> MLSIKDLHVSVEDKAILRGLSLDVHPGEVHAIMGPNGSGKSTLSATLAGREDYEVTGGTVEFKGKDLLALSPEDRAGEGIFMAFQYPVEIPGVSNQFFLQTALNAVRSYRGQETLDRFDFQDLMEEKIALLKMPEDLLTRSVNVGFSGGEKKRNDILQMAVLEPELCILDESDSGLDIDALKVVADGVNSLR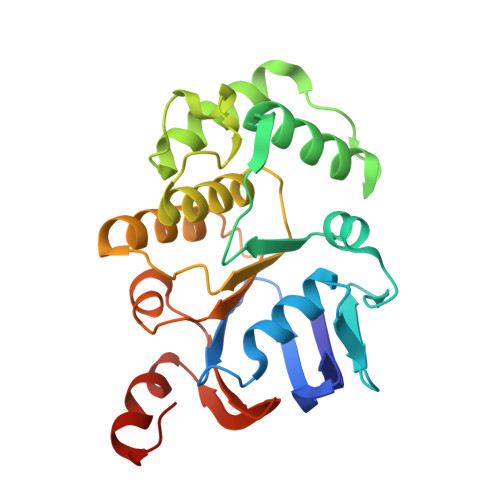DGKRSFIIVTHYQRILDYIKPDYVHVLYQGRIVKSGDFTLVKQLEEQGYGWLTEQQ> MPSASSGYTFADFLRRLERSPDSHMAPLYHEHRELFVRRHDMFARVISSVTWSKGVALVAAAGYTQAVNVTIYRALLARMLLHNRHVRQCGAGSVVPWSAALRTYSEAIATHGNAVPTRMTL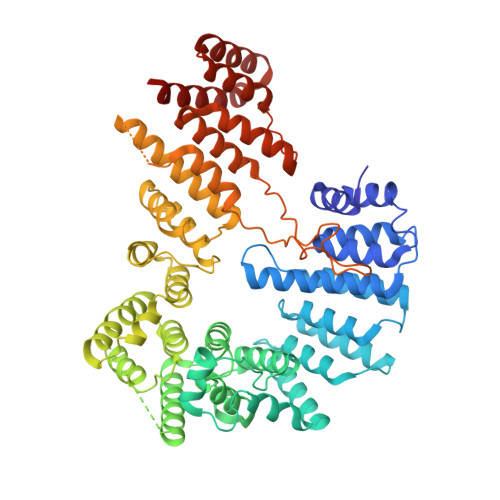SALRLCTPARQWVAAISLLMLSQANDKLTLPMLIDAAGCCATPAAWEKAMALLGRFHAQSLQVLPDSIQSLRPVGTSASTVDAAAHALLPRSEGPTPEQKHILTVINKVVSAVPWQVALSNEMCRSYLTHLVASTTLRPTEKTASLTTAVQQLPWEAFVTLMKTVTATVQEGSQGVLGSRSTPQLPPPQDGMERGDVAKSLLSNSIIREGVNLLQSEPETAIPFITTILYKLPSAEAAALFLSEATSAYRNSSSAVVAAAIRHPVVVGALLKRCADSNSWYLAASIFKSTSPTAIPCDVASDLVIQMRRANQAPLVVDVLQKYIVPSRTKLTEEAIEAALLCVLVHNRALAKASAVVAGTSPDNRTGKPNGIGVANGVHWISALSWATDLLEEGVESRILQTGTTPSVGGVNHEDPTVLLRKKTLSPRILSLLIYICVNAGSPRGGLFALGYARTVSKTELELSEEITALLYCMMYDRPREAESIIQHAVKKHGEYKGKYLGRLLVASQEAKGSALRNQT>HMSTSISEAEPPRVLITGGLGQLGVGLANLLRKRFGKDNVILSDIRKPPAHVFHSGPFVYANILDYKSLREIVVNHRISWLFHYSALLSAVGEANVSLARDVNITGLHN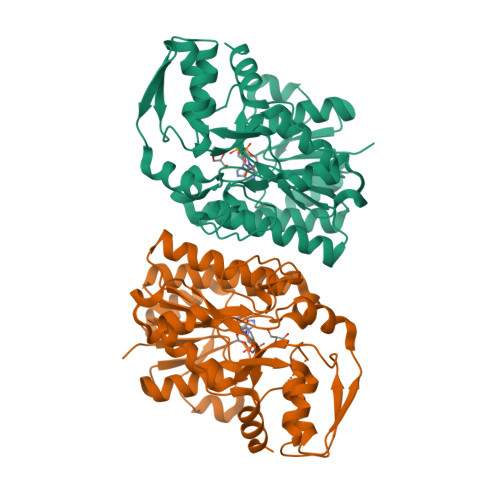VLDVAAEYNVRLFVPSTIGAFGPTSPRNPAPDLCIQRPRTIYGVSKVHTELMGEYYYYRYGLDFRCLRYPGIISADSQPGGGTTDYAVQIFHAAAKNGTFECNLEAGTRLPMMYISDCLRATLEVMEAPAERLSMRTYNISAMSFTPEELAQALRKHAPDFQITYCVDPLRQAIAESWPMILDDSNARKDWGWKHDFDLPELVATMLNFHGVSTRVAQVN[6x]>GAMGFNKILVVAVGNICRSPTGERVLQKLLPNKTVASAGIAAEKSRLIGKPADAMAIEVAKENCVDVENHQSQQLTSALCSQYDLILVMEKGHMEALTQIAPEARGKTMLFGQWIGQKDIPDPYRQSKEAFVHAYQLIDEAAQAW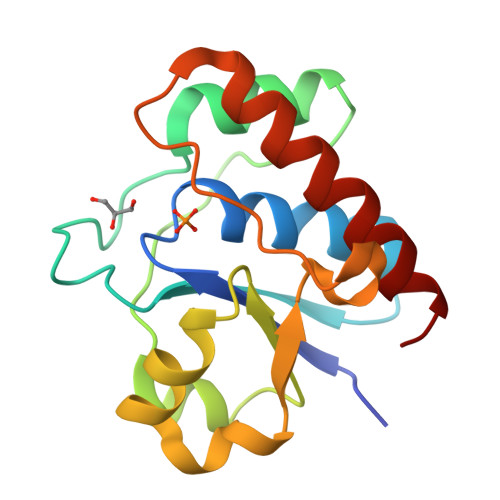AKKL[4x]>MGFCLALAWTLLVGAWTPLGAQNPISWEVQRFDGWYNNLMEHRWGSKGSRLQRLVPASYADGVYQPLGEPHLPNPRDLSNTISRGPAGLASLRNRTVLGVFFGYHVLSDLVSVETPGCPAEFLNIRIPPGDPMFDPDQRGDVVLPFQRSRWDPETGRSPSNPRDPANQVTGWLDGSAIYGSSHSWSDALRSFSRGQLASGPDPAFPRDSQNPLLMWAAPDPATGQNGPRGLYAFGAERGNREPFLQALGLLWFRYHNLWAQRLARQHPDWEDEELFQHARKRVIATYQNIAVYEWLPSFLQKTLPEYTGYRPFLDPSISSEFVAASEQFLSTMVPPGVYMRNASCHFQGVINRNSSVSRALRVCNSYWSREHPSLQSAEDVDALLLGMASQIAEREDHVLVEDVRDFWPGPLKFSRTDHLASCLQRGRDLGLPSYTKARAALGLSPITRWQDINPALSRSNDTVLEATAALYNQDLSWLELLPGGLLESHRDPGPLFSTIVLEQFVRLRDGDRYWFENTRNGLFSKKEIEEIRNTTLQDVLVAVINIDPSALQPNVFVWHKGDPCPQPRQLSTEGLPACAPSVVRDYFEGSGFGFGVTIGTLCCFPLVSLLSAWIVARLRMRNFKRLQGQDRQSIVSEKLVGGMEALEWQGHKEPCRPVLVYLQPGQIRVVDGRLTVLRTIQLQPPQKVNFVLSSNRGRRTLLLKIPKEYDLVLLFNLEEERQALVENLRGALKESGLSIQEWELREQELMRAAVTREQRRHLLETFFRHLFSQVLDINQADAGTLPLDSSQKVREALTCELSRAEFAESLGLKPQDMFVESMFSLADKDGNGYLSFREFLDILVVFMKGSPEEKSRLMFRMYDFDGNGLISKDEFIRMLRSFIEISNNCLSKAQLAEVVESMFRESGFQDKEELTWEDFHFMLRDHNSELRFTQLCVKGVEVPEVIKDLCRRASYISQDMICPSPRVSARCSRSDIETELTPQRLQCPMDTDPPQEIRRRFGKKVTSFQPLLFTEAHREKFQRSCLHQTVQQFKRFIENYRRHIGCVAVFYAIAGGLFLERAYYYAFAAHHTGITDTTRVGIILSRGTAASISFMFSYILLTMCRNLITFLRETFLNRYVPFDAAVDFHRLIASTAIVLTVLHSVGHVVNVYLFSISPLSVLSCLFPGLFHDDGSEFPQKYYWWFFQTVPGLTGVVLLLILAIMYVFASHHFRRRSFRGFWLTHHLYILLYVLLIIHGSFALIQLPRFHIFFLVPAIIYGGDKLVSLSRKKVEISVVKAELLPSGVTHLRFQRPQGFEYKSGQWVRIACLALGTTEYHPFTLTSAPHEDTLSLHIRAAGPWTTRLREIYSAPTGDRCARYPKLYLDGPFGEGHQEWHKFEVSVLVGGGIGVTPFASILKDLVFKSSVSCQVFCKKIYFIWVTRTQRQFEWLADIIREVEENDHQDLVSVHIYITQLAEKFDLRTTMLYICERHFQKVLNRSLFTGLRSITHFGRPPFEPFFNSLQEVHPQVRKIGVFSCGPPGMTKNVEKACQLINRQDRTHFSHHYENF[2x];>MATLGHTFPFYAGPKPTFPMDTTLASIIMIFLTALATFIVILPGIRGKTRLFWLLRVVTSLFIGAAILAVNFSSEWSVGQVSTNTSYKAFSSEWISADIGLQVGLGGVNITLTGTPVQQLNETINYNEEFTWRLGENYAEEYAKALEKGLPDPVLYLAEKFTPRSPCGLYRQYRLAGHYTSAMLWVAFLCWLLANVMLSMPVLVYGGYMLLATGIFQLLALLFFSMATSLTSPCPLHLGASVLHTHHGPAFWITLTTGLLCVLLGLAMAVAHRMQPHRLKAFFNQSVDEDPMLEWSPEEGGLLSPRYRSMADSPKSQDIPLSEASSTKAYYRPRRLSLVPADVRGLAPAALSALPGALLAQAWRALLPGLRC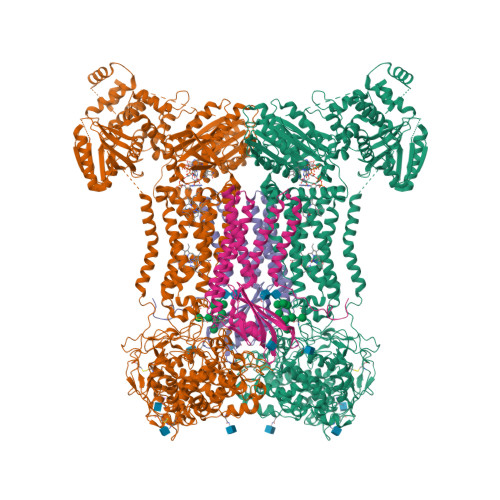PKAGKESRLGPPHSPWRFGPEGCEERWAEHTGDSPRPLRGRGTGRLWRWGSKERRACGVRAMLPRLVSNSGLKRPSCLDLPKCWDYRRDARAFFHLLEPTPCVTSRHTPLI[2x]> MEQRETIMLPGSDYNHWLIVMEFPKDPAPSRDQMIDTYLNTLATVLGSMEEAKKNMYAFSTTTYTGFQCTIDEETSEKFKGLPGVLWVLPDSYIDVKNKDYGGDKYINGEIIPSTYPTYQPKQLEHHHHHHHH;> HMAELRRQGVAPTVVTYNALIDG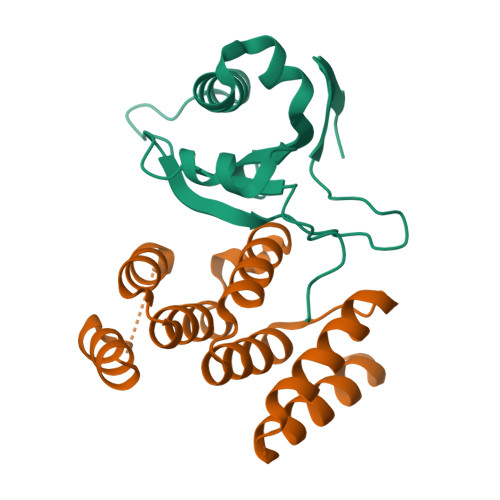LCKAGKLDEALKLFEEMVEKGIKPDEFTFSSVLKACARLGALELGKQIHGYVIKSGFESNVVVYNALIDMYSKCGLLEEARKVFDEMPEKDELTYRRVVESYCRAKRFE>GSMASTQDAVHTDAVQDWKNGTINAQLTLDLARARMRLPADRTAASQFLRYKAPAQLKDVYLSVLVDSQNRVGDCLAHEKIRLADITALVDAGHHAVTTLSPSVRSLQLSHQTPLTALARLFVTHETAYVPAIPPTSAVSRPYTGILIDARGSLPVHGEYVSEPLSACLFPKIWSTDMDLIYEKNMVHPDRAKAWGVVRYGSVWDEKMYRDRIGTTPLKIIARGVFGQQRTDPIIASKDAAQILARPENLRLLAEGNVIILCDEAALRVHVPYPLVDEHFYFAYHDVKRFLTDERSPGVGVRSGINTLKITVYDVRFVANSPEILASEKDRVDVIATALKKMGPYTRFLIEGHTADLHRPQEEAALSVARAQRMAQELSRRGIEMTRITTAGHGATKPIAPSDTHANKAKNRRVEITILRD[2x]

Treponema pallidum subspecies pallidum (hereafter T. pallidum) is a medically important spirochete bacterium and the causative agent of syphilis, a chronic, multistage systemic disease transmitted sexually, through direct contact with an infectious lesion, or in utero. The T. pallidum protein Tp0624 is annotated as belonging to the OmpA-OmpF porin (OOP) family. The C-terminal region of Tp0624 is predicted to adopt an OmpA domain architecture, but it is unclear what role a canonical peptidoglycan binding domain might possess in an organism that contains an unusual form of peptidoglycan and has a divergent cell envelope ultrastructure. Treponema pallidum transcriptomic and proteomic studies have shown that Tp0624 is expressed during infection, yet its precise biological role is unknown.

Further complicating the functional prediction of Tp0624 is the observation that the N-terminal two thirds of the protein does not show significant sequence homology to any functionally- or structurally-characterized protein. The presence of an OmpA-like domain suggests a potential role for Tp0624 in peptidoglycan coordination and cell envelope stabilization, which could be facilitated by the uncharacterized N-terminal region. To gain insight into the function of Tp0624, we first determined its three-dimensional structure, which revealed a trimodular architecture incorporating a highly divergent OmpA-like domain and a previously uncharacterized tandem domain with intriguing implications for peptidoglycan coordination. Moreover, compared to conventional Gram-negative bacteria, T. pallidum has an inherently fragile cell envelope composed of a chemically distinct peptidoglycan layer that is thinner and more spatially separated from the outer membrane, as well as periplasmic flagella (endoflagella) that are located between the outer membrane and the peptidoglycan layer. These ultrastructural differences suggest that treponemes such as T. pallidum may harbor divergent molecular strategies for linking the peptidoglycan layer with the inner and outer membranes to stabilize the bacterial cell envelope. Collectively, these data provide insight into how the unusual cell envelope structure may be stabilized in the human pathogen T. pallidum.>[2x]GPGSMMSLNAAAAADERSRKEMDRFQVERMAGQGTFGTVQLGKEKSTGMSVAIKKVIQDPRFRNRELQIMQDLAVLHHPNIVQLQSYFYTLGERDRRDIYLNVVMEYVPDTLHRCCRNYYRRQVAPPP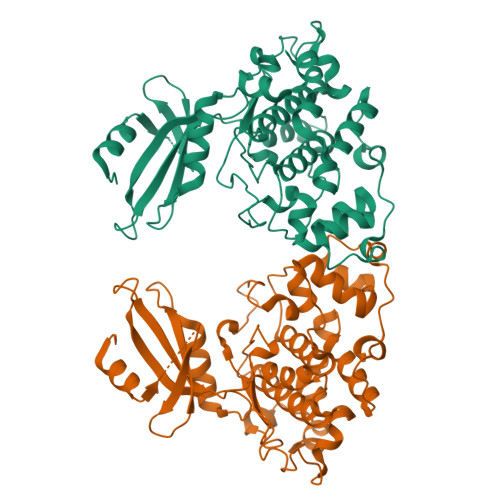ILIKVFLFQLIRSIGCLHLPSVNVCHRDIKPHNVLVNEADGTLKLCDFGSAKKLSPSEPNVAYICSRYYRAPELIFGNQHYTTAVDIWSVGCIFAEMMLGEPIFRGDNSAGQLHEIVRVLGCPSREVLRKLNPSHTDVDLYNSKGIPWSNVFSDHSLKDAKEAYDLLSALLQYLPEERMKPYEALCHPYFDELHDPATKLPNNKDLPEDLFRFLPNEIEVMSEAQKAKLVRK>[4x]AEGTRGRSSTARCSLFGSDFVNTFDGSMYSFAGYCSYLLAGGCQKRSFSIIGDFQNGKRVSLSVYLGEFFDIHLFVNGTVTQGDQRVSMPYASKGLYLETEAGYYKLSGEAYGFVARIDGSGNFQVLLSDRYFNKTCGLCGNFNIFAEDDFMTQEGTLTSDPYDFANSWALSSGEQWCERASPPSSSCNISSGEMQKGLWEQCQLLKSTSVFARCHPLVDPEPFVALCEKTLCECAGGLECACPALLEYARTCAQEGMVLYGWTDHSACSPVCPAGMEYRQCVSPCARTCQSLHINEMCQERCVDGCSCPEGQLLDEGLCVESTECPCVHSGKRYPPGTSLSRDCNTCICRNSQWICSNEECPGECLVTGQSHFKSFDNRYFTFSGICQYLLARDCQDHSFSIVIETVQCADDRDAVCTRSVTVRLPGLHNSLVKLKHGAGVAMDGQDVQLPLLKGDLRIQHTVTASVRLSYGEDLQMDWDGRGRLLVKLSPVYAGKTCGLCGNYNGNQGDDFLTPSGLAEPRVEDFGNAWKLHGDCQDLQKQHSDPCALNPRMTRFSEEACAVLTSPTFEACHRAVSPLPYLRNCRYDVCSCSDGRECLCGALASYAAACAGRGVRVAWREPGRCELNCPKGQVYLQCGTPCNLTCRSLSYPDEECNEACLEGCFCPPGLYMDERGDCVPKAQCPCYYDGEIFQPEDIFSDHHTMCYCEDGFMHCTMSGVPGSLLPDAVLSSPLSHRSKR;>SLSCRPPMVKLVCPADNLRAEGLECTKTCQNYDLECMSMGCVSGCLCPPGMVRHENRCVALERCP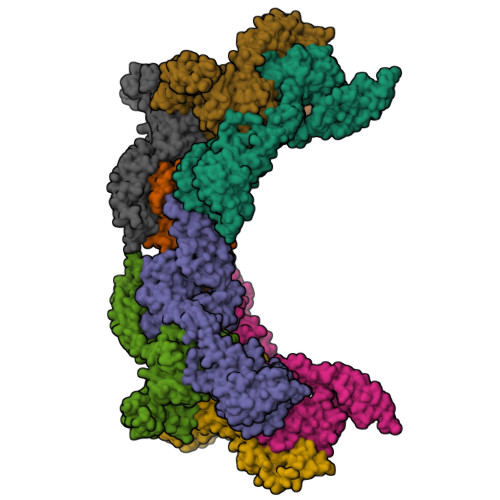CFHQGKEYAPGETVKIGCNTCVCQDRKWNCTDHVCDATCSTIGMAHYLTFDGLKYLFPGECQYVLVQDYCGSNPGTFRILVGNKGCSHPSVKCKKRVTILVEGGEIELFDGEVNVKRPMKDETHFEVVESGRYIILLLGKALSVVWDRHLSISVVLKQTYQEKVCGLCGNFDGIQNNDLTSSNLQVEEDPVDFGNSWKVSSQCADTRKVPLDSSPATCHNNIMKQTMVDSSCRILTSDVFQDCNKLVDPEPYLDVCIYDTCSCESIGDCACFCDTIAAYAHVCAQHGKVVTWRTATLCPQSCEERNLMENGYECMWRYNSCAPACQVTCQHPEPLACPVQCVEGCHAHCPPGKILDELLQTCVDPEDCPVCEVAGRRFASGKKVTLNPSDPEHCQICHCDVVNLTCEACQEPGGLVVPPHHHHHH[4x]> MIRGKLLLPEKKVVFINESEVQSLRKDVVDALKVFSSLACELADNNETKATNIFADLISMIYKLPMLISYVPSDKLSTPHEYFFAYIVFRHLVEDSMPSNDIAKLLEILEEKKRDEIKEVLDYARTLRKIYEKLLYVPADTRPGYNFTSLASHLQLSSILVWLLQKGSVDLNYLRISALLHDIGKLFNPTNHVSESIKILDEVIEGSECLKTNLSRVKSLVEQHHAPLETILNDADRLAASTDRFSEIVKGALNNTKIGECYSLCYGRDVRTKECMECLEEYGEETYSEESKRLYDVISNSVVSQKVEGNAIGYLVYIDFPGIQRFITSFPKLREMSFASFLVDFVTSIYSFIVLDQAYYERTGKKSRIPAEALLSGYGGHSYIIVRSDFGSKDEVKAWLESVSSSALSKLGIRLDVKVADFAYENYVRNYKEVYEDMMSKSYERYLIRDEGKVYSYGLHRVCDNCGIRPAVNRSDDGEYLCETCNLVRDLSKNRGFIAKYKSKYTLYEEQRIEISPKEDIKFKLDKNQDPTSYAMEIIAGYRTTSDSRYIALIKADGNNAGKIFGNTVTFSEYVDKSFRLDF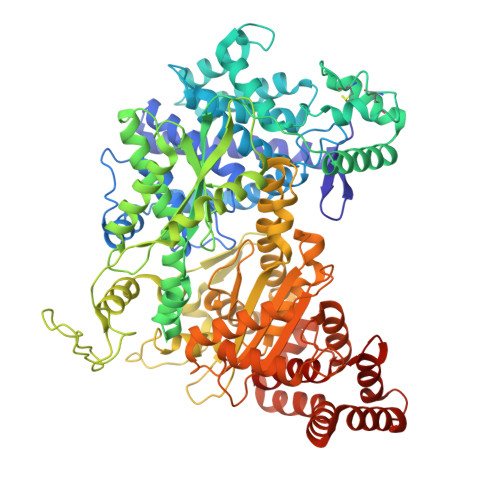GVKKMFYDTLLDIMRASSDESIKKDLVSRILLGVLYLGGDDIMLLSPSAIAVPFAVKMFKRSLEYTGFTFKVGIISVKPDHPVQFAYGAVNALMEESKIHTGEKSSIGVLVFSSTLASEGVVKSDLKNYRKEKESFLVVSNDVDDVERLLNLMELDDFGKLMELYWNPEEGRKVIRDKIRSLERFVNYADTHDFYNTLAYLIRSKAKSEENSLIKRIIDLTIKGRDDFVFPLYDYYFILKSIRVGI> GPMQEAAVREPQIFFNLTYTEYLDKVAASHGSPPDKSDLPWNDTMGSFPGNETDDGVQTETGSSLSRRGHIVNLRKREPFGEESRNDRVTQDMLQALHDLCVERFGTGYRAVSGLCYTDRRATRKIECNKPSVRERDRSVTRACPKGQECTTFNAYN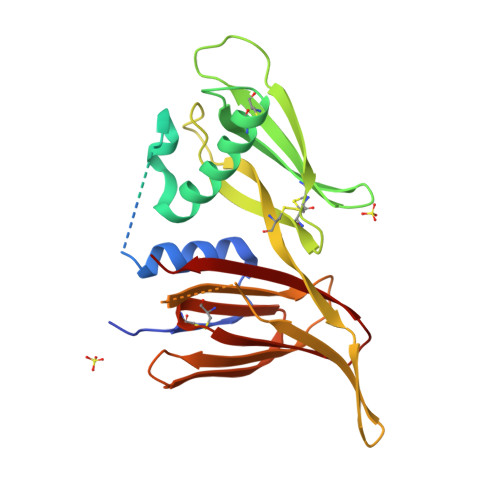FRNRHHQVTFPVCGPRIEVKDRHDIGIHTEWQGTWYPESPKSPGTYDYFAQMAGTLNGYFGYDGVYSDGYKTSSHGYGHSWSCINCPRGKVTITNTYRATWAFGYTSPHS> 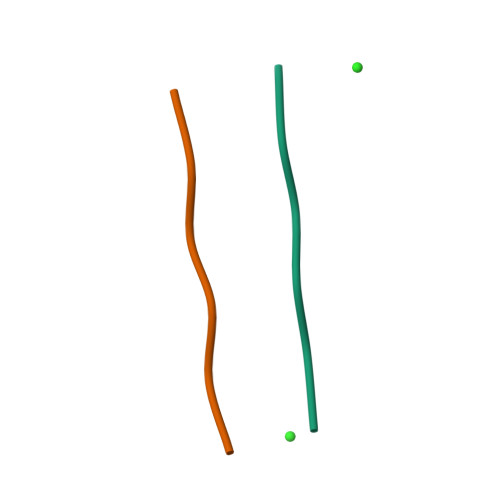NFLVHS N-[(2R)-10-hydroxy-2,7-dimethyl-1,2,3,4-tetrahydropyrido[1,2-b]indazol-2-yl]-4-(4H-1,2,4-triazol-4-yl)benzamide 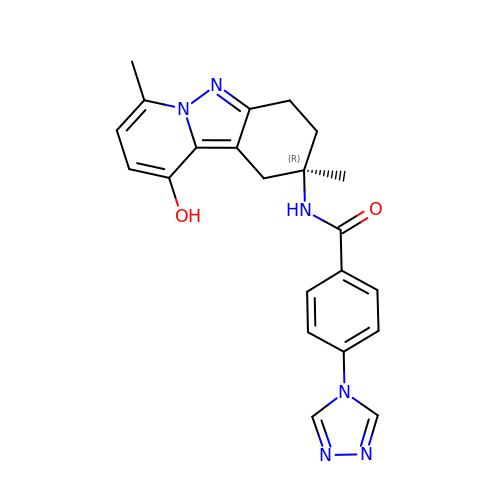| C22 H22 N6 O2 | GHULVZIKWFGNRE-JOCHJYFZSA-N>[2x]MNPLAPELGEVARFAMLASQAITTTSGSAIVDG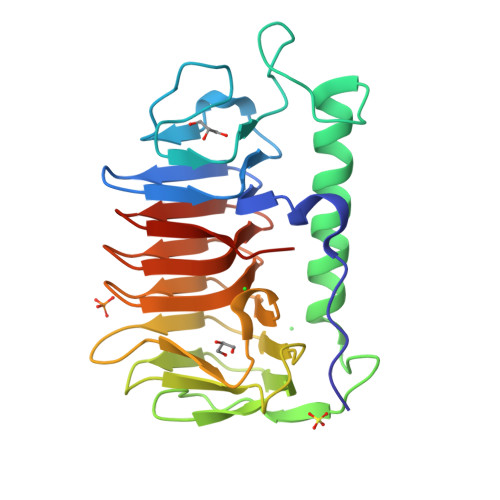DLGILDQARSYYAGFTPGVNAGEFDELTNGLSYAGDDSTPPYVVPVPYASMVAFINQSRTDLGIAYNFLAADPNPNAATQVCPIELGNLTLTRGVYKTAADVTLQTGTLTLDGEGDPDSVFIFTIGGNLTSGAPGGDIVLINGAQAKNIYWRTAGKTVIGTNTNFSGNVFAWSEVNVRTGANVTGRLFAVTDQVTLDANAVTKANLEHHHHHH>MSAIENFDAHTPMMQQYLRLKAQHPEILLFYRMGDFYELFYDDAKRASQLLDISLTKRGASAGEPIPMAGIPYHAVENYLAKLVNQGESVAICEQIGDPATSKGPVERKVVRIVTPGTISDEALLQERQDNLLAAIWQDSKGFGYATLDISSGRFRLSEPADRETMAAELQRTNPAELLYAEDFAEMSLIEGRRGLRRRPLWEFEIDTARQQLNLQFGTRDLVGFGVENAPRGLCAAGCLLQYAKDTQRTTLPHIRSITMEREQDSIIMDAATRRNLEITQNLAGGAENTLASVLDCTVTPMGSRMLKRWLHMPVRDTRVLLERQQTIGALQDFTAGLQPVLRQVGDLERILARLALRTARPRDLARMRHAFQQLPELRAQLETVDSAPVQALREKMGEFAELRDLLERAIIDTPPVLVRDGGVIASGYNEELDEWRALADGATDYLERLEVRERERTGLDTLKVGFNAVHGYYIQISRGQSHLAPINYMRRQTLKNAERYIIPELKEYEDKVLTSKGKALALEKQLYEELFDLLLPHLEALQQSASALAELDVLVNLAERAYTLNYTCPTFIDKPGIRITEGRHPVVEQVLNEPFIANPLNLSPQRRMLIITGPNMGGKSTYMRQTALIALMAYIGSYVPAQKVEIGPIDRIFTRVGAADDLASGRSTFMVEMTETANILHNATEYSLVLMDEIGRGTSTYDGLSLAWACAENLANKIKALTLFATHYFELTQLPEKMEGVANVHLDALEHGDTIAFMHSVQDGAASKSYGLAVAALAGVPKEVIKRARQKLRELESISPNAA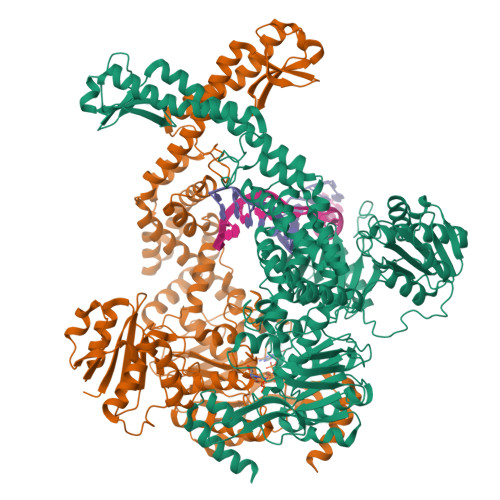ATQVDGTQMSLLSVPEETSPAVEALENLDPRSLTPRQALEWIYRLKSLV[2x]>[2x]MTKYRLSEGPRAFTYQVDGEKKSVLLRQVIAVTDFNDVKAGTSGGWVDADNVLSQQGDC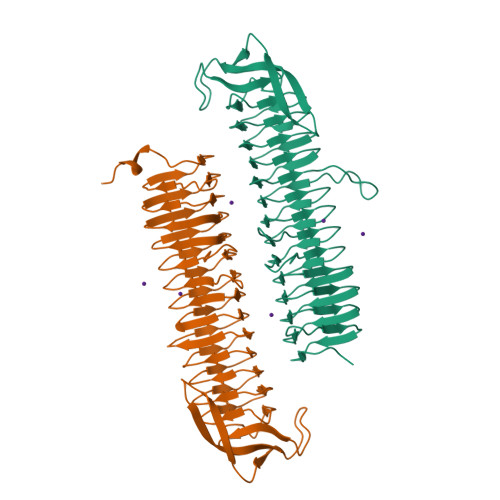WIYDENAMAFAGTEITGNARITQPCTLYNNVRIGDNVWIDRADISDGARISDNVTIQSSSVREECAIYGDARVLNQSEILAIQGLTHEHAQILQIYDRATVNHSRIVHQVQLYGNATITHAFIEHRAEVFDFALIEGDKDNNVWICDCAKVYGHARVIAGTEEDAIPTLRYSSQVAEHALIEGNCVLKHHVLVGGHAEVRGGPILLDDRVLIEGHACIQGEILIERQVEISGRAAVIAFDDNTIHLRGPKVINGEDRITRTPLVGSLLEHHHHHH>MNKTYAACPQNWIGVENKCFYFSEYPSNWTFAQAFCMAQEAQLARFDNQDELNFLMRYKANFDSWIGLHRESSEHPWKWTDNTEYNNTIPIRGEERFAYLNNNGISSTRIYSLRMWICSKLNAS[16x];>TGSAKLECPQDWLSHRDKCFHVSQVSNTWKEGRIDCDKKGATLLLIQDQEELRFLLDSIKEKYNSFWIGLSYTLTDMNWKWINGTAFNSDVLKITGVTENGSCAAISGEKVTSEGCSSDNRWICQKELNGTHHHHHH[8x]

In mice, the NKR-P1 family consists of five members, which include three stimulatory (NKR-P1A, NKR-P1C, and NKR-P1F) and two inhibitory (NKR-P1B and NKR-P1G) members. Of these, NKR-P1B, NKR-P1F, and NKR-P1G recognize host-encoded Clr molecules, which like their receptor counterparts are C-type lectin-related type II transmembrane proteins that form disulfide-linked dimers via cysteine residues within their membrane-proximal stalks. While the expression of most Clr molecules is tissue-specific, Clr-b transcripts have been identified in most tissues except brain, suggesting this molecule may represent a broad marker of healthy-self. Indeed, downregulation of Clr-b has been implicated in missing-self recognition of virally infected, cancerous, and allogeneic cells.

To understand the molecular basis underpinning recognition of Clr-b by NKR-P1B, we expressed their corresponding CTLDs and determined the structure of the co-complex to 2.9 Å resolution. The crystallographic asymmetric unit comprised eight protomers of NKR-P1B and sixteen protomers of Clr-b, which together formed eight highly similar NKR-P1B:Clr-b complexes (root mean square deviation (r.m.s.d) ~ 0.5 Å overall Cα atoms). NKR-P1B engaged Clr-b via a head-to-head docking mode such that the N-terminus of each molecule protruded from opposite ends of the complex. Surprisingly, a single NKR-P1B protomer engaged one half of the Clr-b homodimer, making contacts exclusively with only one Clr-b monomer. This unusual trimeric 1 NKR-P1B: 2 Clr-b stoichiometry was conserved in all eight of the complexes present within the crystallographic asymmetric unit, and differs from the 2:2 stoichiometry observed for the related human NKp65:KACL complex, despite similarities in overall docking mode. Unlike Clr-b, NKR-P1B was not observed to form a classic homodimer, most likely due to the orientation of the α2-helix, which protruded in a fashion that would sterically clash with a neighboring NKR-P1B protomer. Instead, two symmetry-related NKR-P1B molecules packed together to form a distinct non-classic homodimer. Within the crystal, two trimeric NKR-P1B:Clr-b complexes were bridged via an NKR-P1B dimer to produce a hexameric arrangement Here, each of the Clr-b N-termini lay planar to each other, indicating that these molecules could potentially be arranged in cis within a single target cell membrane. NKR-P1B and Clr-b interacted via an imperfect interface that was modest in size, burying a total solvent accessible surface area of 1450 Å2, and characterized by poor shape complementarity ((Sc) = 0.55, where 1 indicates a geometrically perfect fit).> QYSPNTQQGRTSIVHLFEWRWVDIALECERYLAPKGFGGVQVSPPNENVAIYNPFRPWWERYQPVSYKLCTRSGNEDEFRNMVTRCNNVGVRIYVDAVINHMC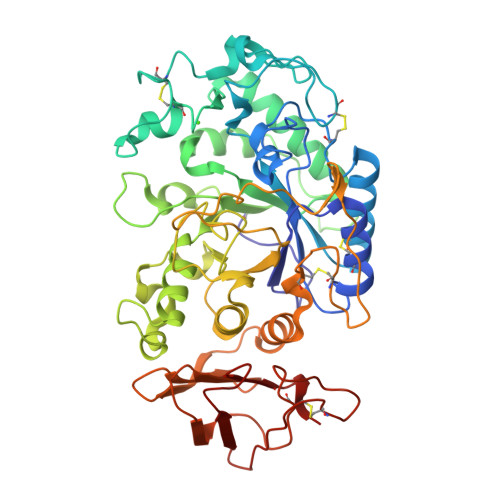GNAVSAGTSSTCGSYFNPGSRDFPAVPYSGWDFNDGKCKTGSGDIENYNDATQVRDCRLTGLLDLALEKDYVRSKIAEYMNHLIDIGVAGFRLDASKHMWPGDIKAILDKLHNLNSNWFPAGSKPFIYQEVIDLGGEPIKSSDYFGNGRVTEFKYGAKLGTVIRKWNGEKMSYLKNWGEGWGFVPSDRALVFVDNHDNQRGHGAGGASILTFWDARLYKMAVGFMLAHPYGFTAVMSSYRWPRQFQNGNDVNDWVGPPNNNGVIKEVTINPDTTCGNDWVCEHRWRQIRNMVIFRNVVDGQPFTNWYDNGSNQVAFGRGNRGFIVFNNDDWSFSLTLQTGLPAGTYCDVISGDKINGNCTGIKIYVSDDGKAHFSISNSAEDPFIAIHAESKL>[2x]MGHHHHHHGSTELTPDQQTLLHFIMDSYNKQRMPQEITNKILKEAFSAEENFLILTEMATNHVQVLVEFTKKLPGFQTLDHEDQIALLKGSAVEAMFLRSAEIFNKKLPSGHSDLLEARIRNSGISDEYITPMFSFYKSIGELKMTQEEYALLTAIVILSPDRQYIKDREAVEKL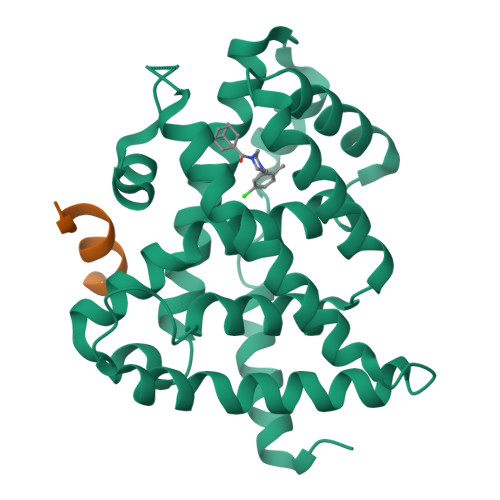QEPLLDVLQKLCKIHQPENPQHFACLLGRLTELRTFNHHHAEMLMSWRVNDHKFTPLLCEIWDVQ;>[2x]KDHQLLRYLLDKDE> MAVKKIAIFGATGQTGLTTLAQAVQAGYEVTVLVRDSSRLPSEGPRPAHVVVGDVLQAADVDKTVAGQDAVIVLLGTRNDLSPTTVMSEGARNIVAAMKAHGVDKVVACTSAFLLWDPTKVPPRLQAVTDDHIRMHKVLRESGLKYVAVMPPHIGDQPLTGAYTVTLDGRGPSRVISKHDLGHFMLRCLTTDEYDGHSTYPSHQYQ

Biliverdin Reductase B (BLVRB) is an NADPH-dependent reductase that catalyzes the reduction of multiple substrates and is therefore considered a critical cellular redox regulator. However, it was later discovered that BLVRB is identical to flavin reductase (FR) that is a promiscuous enzyme responsible for reduction of flavin substrates, which includes flavin adenine dinucleotide (FAD) and flavin mononucleotide (FMN). Structurally, BLVRB comprises a typical SDR fold with a central β-sheet flanked α-helices on each side. Like other SDR family members, the coenzyme binding site is within the conserved SDR fold itself, while substrate specificity is dictated by the variable C-terminal lobe.

In an effort to identify the conformational changes within BLVRB necessary to facilitate coenzyme binding, we have solved the first X-ray crystal structures of apo human BLVRB that has eluded crystallization until now. At the cofactor binding site, three arginines show clear remodeling compared to the holo state. In both apo-RT and apo-cryo structures, R35 and R39 are both found in specific conformations, as indicated by clear electron density. Most surprising is that in the apo-cryo structure, the R78-loop (residues 77–80), which exhibits high R1 relaxation rates indicative of disorder in solution, is well modelled in electron density where the R78 sidechain interacts with its crystallographic mate (not shown). Although this suggests that the R78-loop is “closed” and would therefore block binding and release of the coenzyme, the R78 side chain does not form the hydrogen bond to T12 CO that forms the clamp. To determine if this defined conformation of the R78-loop is an artifact of cooling to cryogenic temperatures, the complementary room-temperature (20 °C) structure was compared. One important difference between the apo BLVRB structures was that the apo-cryo structure exhibited a defined density of the R78-loop that would block coenzyme entry and release, while this region was disordered in the apo-RT structure that would facilitate such an interaction. Such comparisons highlight the potential misinterpretation of structures determined by cryogenic crystallography without complementary ambient temperature experiments. Elsewhere, both apo structures are generally similar, but there are significant regions throughout the enzyme which differ when comparing the apo-structures and the previously determined holo-structure (0.8 Å all-atom RMSD). Specifically, loops 34–46, 115–126, and 153–176 show large displacements and conformational changes with some regions having greater than a 2 Å Cα RMSD.> GAMAKVQVNNVVVLDNPSPFYNPFQ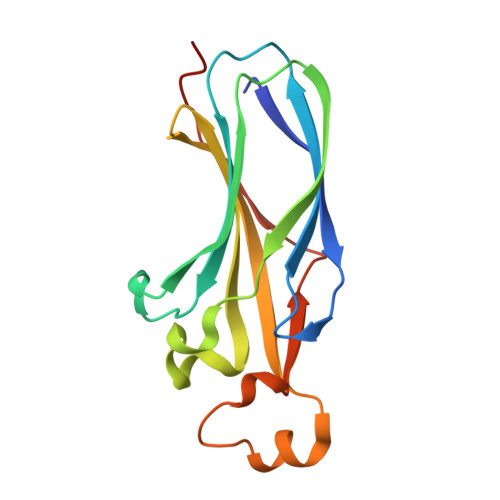FEITFECIEDLSEDLEWKIIYVGSAESEEYDQVLDSVLVGPVPAGRHMFVFQADAPNPGLIPDADAVGVTVVLITCTYRGQEFIRVGYYVNNEYTETELRENPPVKPDFSKLQRNILASNPRVTRFHINWEDN> M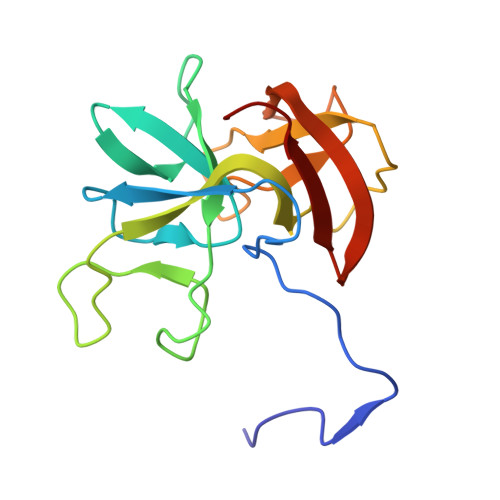AFNNAVLQEVSDLPAGEVIKASPHNVSAFEVFQNGLIEGRFVKFDAGSIDILDASATPTIAGIAKRKVTGEIGPGVYSTSGIEIDQVAEVINFGFATVTVQDAAAPSKYDPVYAINLDSAEAGKATENSGATGALAVADCVFWEQKAANVWLVRMNKFL The fixation of kinetically inert atmospheric dinitrogen (N2) to ammonia (NH3) is catalyzed in some specific microbes by a single family of enzymes known as nitrogenases, with turnover frequencies of around one N2 fixed per second and a second-order rate constant of ∼104 M–1 s–1 (kcat/KM).1−6 The Mo-dependent nitrogenase consists of an N2-reducing molybdenum-iron (MoFe) protein and a corresponding reductase called the iron (Fe) protein. The MoFe protein is a ∼230 kDa (αß)2 heterotetramer (NifDK), where each αß half contains an electron-transferring [8Fe–7S] P cluster and a [7Fe–9S–C–Mo]/homocitrate FeMo cofactor (FeMoco). The Fe protein is a homodimeric NifH2 protein of ∼66 kDa containing a single [4Fe–4S] cluster and two MgATP binding sites. The substrate-reducing proteins of all nitrogenases (MoFe, VFe, and FeFe) are organized as α2ß2(γ2) multimers with two functional halves.

To achieve this, we employed a MoFe protein mutant possessing a single solvent-exposed Cys residue in proximity to the P cluster (α-C45A/L158C, NifD = α); this mutant was previously employed to conjugate a Ru-based photosensitizer in the place of the Fe protein, enabling photo-excited electron transfer to the P cluster. X-ray crystallography confirms the solvent accessibility (albeit somewhat geometrically hidden) of this cysteine residue. The α-L158C mutation is positioned at the Fe protein-binding interface on the MoFe protein. Residue α-L158 is located at the Fe:MoFe protein interface, and we therefore hypothesized that the functionalization of a Cys residue in this location with a steric inhibitor could prevent access of the Fe protein (and, therefore, nitrogenase catalysis). The structure was refined to a resolution of 3.03 Å and contained 2 MoFe proteins in the asymmetric unit. The cell dimensions did not fit any of the previously solved structures and might be due to the introduced mutations that impacted the crystal packing. The α-C45A/L158C MoFe protein was found to overlay well with high-resolution structures previously reported for wild-type MoFe protein from A. vinelandii, suggesting a minimal impact of the introduced mutations on the overall conformation of the MoFe protein. Despite the rather low resolution, some distinct changes in the rotamers of amino acids around the introduced mutations were also observed, once again being consistent with the mutations having been successfully introduced. Importantly, the P cluster and FeMoco of the α-C45A/L158C MoFe protein were both found to be present and intact. A Strep-inhibition reaction was performed on a larger batch of α-C45A/L158C MoFe protein (∼18 mg of Strep-inhibited protein obtained) to evaluate Michaelis–Menten kinetic parameters and the distribution of electrons toward N2 fixation under a range of N2 partial pressures.

>[4x]MTHHHHHHHHGMSREEVESLIQEVLEVYPEKARKDRNKHLAVNDPAVTQSKKAIISNKKSQPGLMTIRGCAYAGSKGVVWGPIKDMIHISHGPVGCGQYSRAGRRNYYIGTTGVNAFVTMNFTSDFQEKDIVFGGDKKLAKLIDEVETLFPLNKGISVQSECPIGCIGDDIESVSKVKGAELSKTIVPVRCEGFRGVSQSLGHHIANDAVRDWVLGKRDEDTTFASTPYDVAIIGDYNIGGDAWSSRILLEEMGLRCVAQWSGDGSISEIELTPKVKLNLVHCYRSMNYISRHMEEKYGIPWMEYNFFGPTKTIESLRAIAAKFDESIQKKCEEVIAKYKPEWEAVVAKYRPRLEGKRVMLYIGGLRPRHVIGAYEDLGMEVVGTGYEFAHNDDYDRTMKEMGDSTLLYDDVTGYEFEEFVKRIKPDLIGSGIKEKFIFQKMGIPFRQMHSWDYSGPYHGFDGFAIFARDMDMTLNNPCWKKLQAPWEASEGAEKVAASA;>[4x]MSQQVDKIKASYPLFLDQDYKDMLAKKRDGFEEKYPQDKIDEVFQWTTTKEYQELNFQREALTVNPAKACQPLGAVLCALGFEKTMPYVHGSQGCVAYFRSYFNRHFREPVSCVSDSMTEDAAVFGGQQNMKDGLQNCKATYKPDMIAVSTTCMAEVIGDDLNAFINNSKKEGFIPDEFPVPFAHTPSFVGSHVTGWDNMFEGIARYFTLKSMDDKVVGSNKKINIVPGFETYLGNFRVIKRMLSEMGVGYSLLSDPEEVLDTPADGQFRMYAGGTTQEEMKDAPNALNTVLLQPWHLEKTKKFVEGTWKHEVPKLNIPMGLDWTDEFLMKVSEISGQPIPASLTKERGRLVDMMTDSHTWLHGKRFALWGDPDFVMGLVKFLLELGCEPVHILCHNGNKRWKKAVDAILAASPYGKNATVYIGKDLWHLRSLVFTDKPDFMIGNSYGKFIQRDTLHKGKEFEVPLIRIGFPIFDRHHLHRSTTLGYEGAMQILTTLVNSILERLDEETRGMQATDYNHDLVR>MAHHHHHHMSEAKRLAAEKAIEYVEDGMIVGVGTGSTVAYFIDALARIQHRIKGAVSSSEQSTARLKQHGIEVIELNHSGNLSLYVDGADECDANKCLIKGGGAALTREKIIAEASERFICIIDPSKQVPVLGRFPLPVEVIPMARSLVARQIRD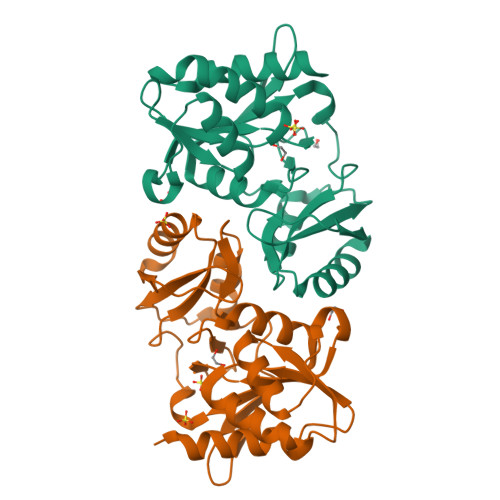MTGGQPTWREGVVTDNGNQILDIHNLQITDPEKLERELNQLPGVVCVGLFARRRADVVIVGGEPPVVL[2x]>MGKLDKASKLIDEENKYYARSARINYYNLVIDHAHGATLVDVDGNKYIDLLASASAINVGHTHEKVVKAIADQAQKLIHYTPAYFHHVPGMELSEKLAKIAPGNSPKMVSFGNSGSDANDAIIKFARAYTGRQYIVSYMGSYHGSTYGSQTLSGSSLNMTRKIGPMLPSVVHVPYPDSYRTYPGETEHDVSLRYFNEFKKPFESFLPADETACVLIEPIQGDGGIIKAPEEYMQLVYKFCHEHGILFAIDEVNQGLGRTGK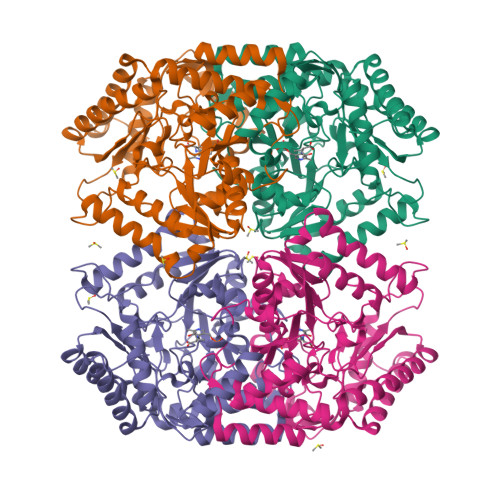MWAIQQFKDIEPDLMSVGKSLASGMPLSAVIGKKEVMQSLDAPAHLFTTAGNPVCSAASLATLDVIEYEGLVEKSATDGAYAKQRFLEMQQRHPMIGDVRMWGLNGGIELVKDPKTKEPDSDAATKVIYYAFAHGVVIITLAGNILRFQPPLVIPREQLDQALQVLDDAFTAVENGEVTIPKDTGKIGW[4x]> MIISEFDRNNPVLKDQLSDLLRLTWPEEYGDSSAEEVEEMMNPERIAVAAVDQDELVGFIGAIPQYGITGWELHPLVVESSRRKNQIGTRLVNYLEKEVASRGGITIYLGTDDLDHGTTLSQTDLYEH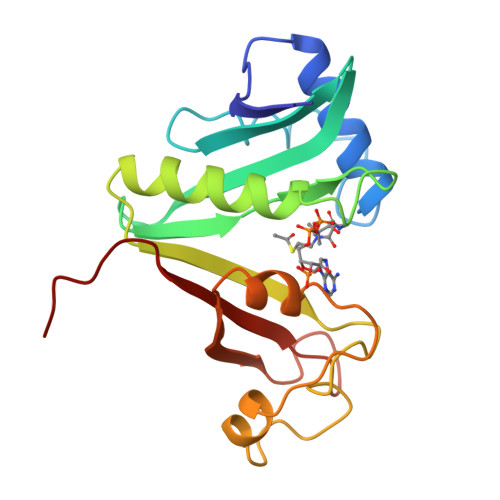TFDKVASIQNLREHPYEFYEKLGYKIVGVLPNANGWDKPDIWMAKTIIPRPDS EICOSANE | 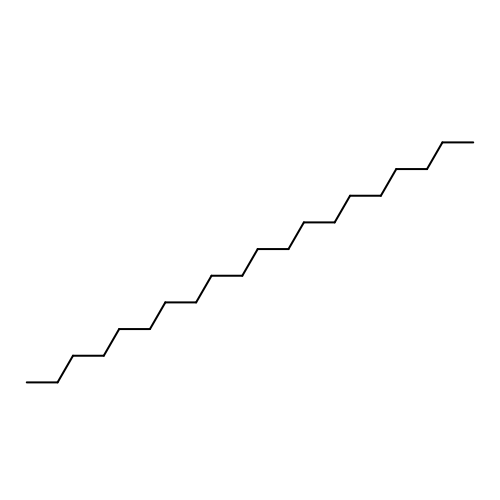C20 H42 | CBFCDTFDPHXCNY-UHFFFAOYSA-N> AIWILIT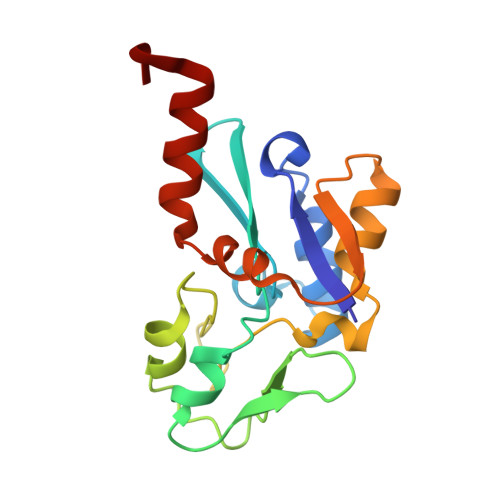PDKCSGCRLCEVTCSLEHEGIIWPEASRIRVFELFPGINVPHTCVQCPDYPCVNACPTNALSVDEKTGAVVVNEEKCITCGACVLACPGKVPRIPAGKGSVVICDLCGGNPKCVEICHEAGHDALKIVTGNYRPIYRTFAKDPQEKSLDIARKVFGEDF> GSMADEATRRVVSEIPVLKTNAGPRDRELWVQRLKEEYQSLIRYVENNKNADNDWFRLESN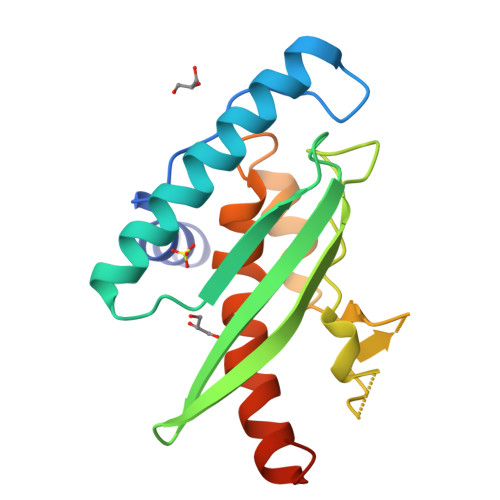KEGTRWFGKCWYIHDLLKYEFDIEFDIPITYPTTAPEIAVPELDGKTAKMYRGGKICLTDHFKPLWARNVPKFGLAHLMALGLGPHLAVEIPDLIQKGVIQHKEKCNQ> AHHHHHHGSSEKACRHC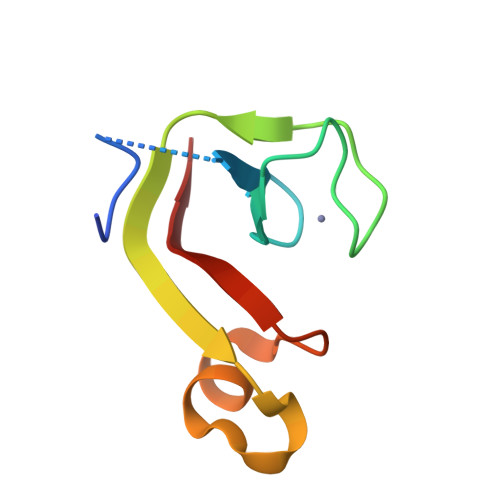HYITSEDRCPVCGSRDLSEEWFDLVIIVDVENSEIAKKIGAKVPGKYAIRVR C-di-GMP is synthesized from guanosine triphosphate by diguanylate cyclase (DGC) enzymes and hydrolyzed to 5′-phosphoguanylyl-(3′ → 5′)-guanosine by c-di-GMP-specific phosphodiesterases (PDEs). CdgH also plays a major role in c-di-GMP synthesis by responding to the presence of bile acids. Here, we reported the crystal structure of the periplasmic portion of V. Cholerae CdgH. Our structure indicated that both tandem PBPb domains of CdgH contain a typical interlobe ligand-binding structural architecture.

Additionally, the two tandem PBPb domains are stably connected through the packing of the C-terminal portion of the α8 helix in lobe-I of the PBPb-I domain with the α7′ helix in lobe-I′ of the PBPb-II domain, placing the two domains perpendicular to each other. Interestingly, the electron density omit map indicated the presence of additional density positions in a deep cleft formed by the two lobes of the PBPb-I domain. The length and shape of the density correspond to an L-arginine molecule, and isothermal titration calorimetry (ITC) experiments confirmed a very strong binding affinity of L-arginine with the tandem PBPb domains (Kd = 1.21 × 10−9 M). The interlobe ligand-binding pocket agrees with many other reported bacterial ligand-binding structures. However, we observed no similar density in the PBPb-II domain, indicating that the PBPb-I domain of our structure is in a ligand-binding conformation, and the PBPb-II domain is in a ligand-free conformation. In the PBPb-I domain bound with L-arginine, the key residues involved in hydrophilic interactions with L-arginine are E56 on the β1-α1 loop, T104 on the β3-α3 loop, R109 on the α3 helix, and E122 on the β5 strand. Additionally, the L-arginine side chain (NH1 And NH2) forms two salt bridges with E56 and E122. In addition to the hydrophilic interactions, the L-arginine side chain is sandwiched by two hydrophobic aromatic rings from F85 and Y148. In the CdgH PBPb-I domain, the α-amino group and the arginine side chain also interacted with E122, which was not observed in other complexes. Structural superposition of the PBPb-I and -II domains revealed that the L-arginine liganded PBPb-I domain adopts a more closed state compared with the unliganded PBPb-II domain. In the type I dimer, the lobe-II′ of the PBPb-II domain of each protomer interacts with the hinge region of the PBPb-I domain of the opposing protomer, revealing a dimerization mode requiring both tandem PBPb domains.

> ATSTTYKVATEADDVVTRVLFDSIAHHFNLEIEYVNYPSFNDILVAIETGNADFAANITYTDLRAQRFDFSRPTNIEYTYLYSYGGLRLPELRLVGIPKGTTYGTLLKEHYPYIQQVEYEGHLEALTLLESGRVDGVVDAINQLKPMLLKGLDVQLLNDQLPIQPVSIVTPKGKHSALLGKIEKYAHSAHVQRLLRESIQKYQLDIRKQALRQSVVESGLNVQRVLRVKLENNPQYALYQPDGSVRGISADVVFQACEMLLLKCELVSNGQETWESMFDDLQDKSIDILAPITVSQQRKNLAYFSESYYHPQAILVKREHYKDDVYSNVSELVAERIGVIKDDFFEELLQQMLPNKILFSYASQEEKVQALLNKEVDYIVLNRANFNLLLRESTEMLPIVEDTMIGSFYQYDIAIGFAKNPLGATLAPLFSRAIKMLNTEQIIHTY>GLDNELSLVDGQDRTLTVQQWDTFLNGVFPLDRNRLTREWFHSGRAKYIVAGPGADEFEGTLELGYQIGFPWSLGVGINFSYTTPNILIDDGDITRPPFGLNSVITPNLFPGVSISADLGNGPGIQEVATFSVDVSGAEGGVAVSNAHGTVTGAA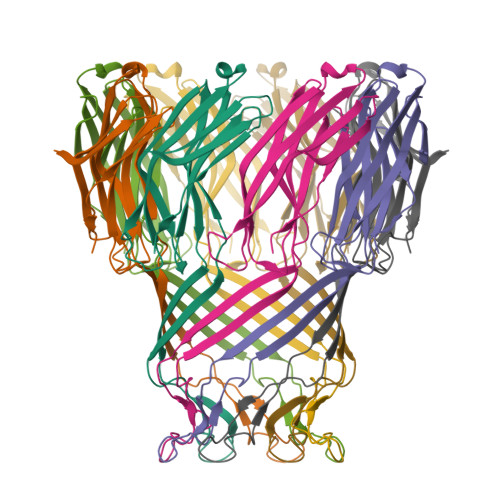GGVLLRPFARLIASTGDSVTTYGEPWNMN[2x]> SPNSQYLKTRILDIYTPEQRAGIEKSEDWRQFSRRMDTHFPKLMNELDSVYGNNEALLPMLEMLLAQAWQSYSQRNSSLKDIDIARENNPDWILSNKQVGGVCYVDLFAGDLKGLKDKIPYFQELGLTYLHLMPLFKCPEGKSDGGYAVSSYRDVNPALGTIGDLREVIAALHEAGISAVVDFIFNHTSNEHEWAQRCAAGDPLFDNFYYIFPDRRMPDQYDRTLREIFPDQHPGGFSQLEDGRWVWTTFNSFQWDLNYSNPWVFRAMAGEMLFLANLGVDILRMDAVPLIWKQMGT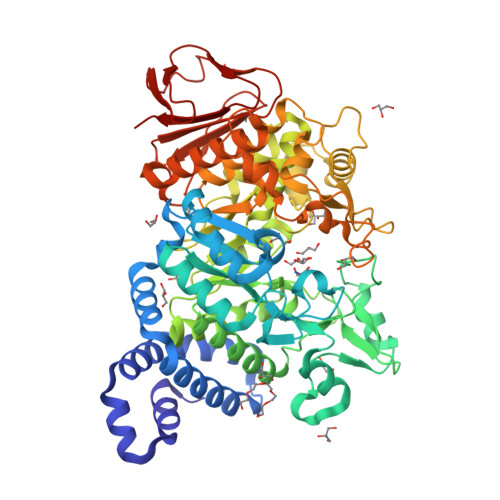SCENLPQAHALIRAFNAVMRIAAPAVFFKSEAIVHPDQVVQYIGQDECQIGYNPLQMALLWNTLATREVNLLHQALTYRHNLPEHTAWVNYVRSHDDIGWTFADEDAAYLGISGYDHRQFLNRFFVNRFDGSFARGVPFQYNPSTGDCRVSGTAAALVGLAQDDPHAVDRIKLLYSIALSTGGLPLIYLGDEVGTLNDDDWSQDSNKSDDSRWAHRPRYNEALYAQRNDPSTAAGQIYQDLRHMIAVRQSNPRFDGGRLVTFNTNNKHIIGYIRNNALLAFGNFSEYPQTVTAHTLQAMPFKAHDLIGGKTVSLNQDLTLQPYQVMWLEIA> APQFFNIIDGSPLNFDDAMEEGRDTEAVKHFLETGENVYNEDPEILPEAEELYAGMCSGCHGHYAEGKIGPGLNDAYWTYPGNETDVGLFS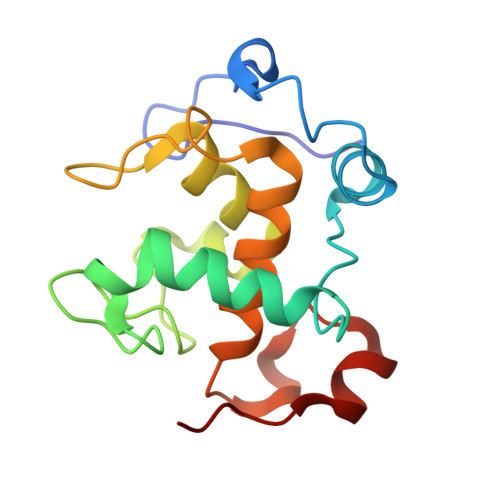TLYGGATGQMGPMWGSLTLDEMLRTMAWVRHLYTGDPKDASWLTDEQKAGFTPFQP5-acetamido-2,6-anhydro-3,5,8-trideoxy-3-fluoro-D-threo-L-galacto-nononic 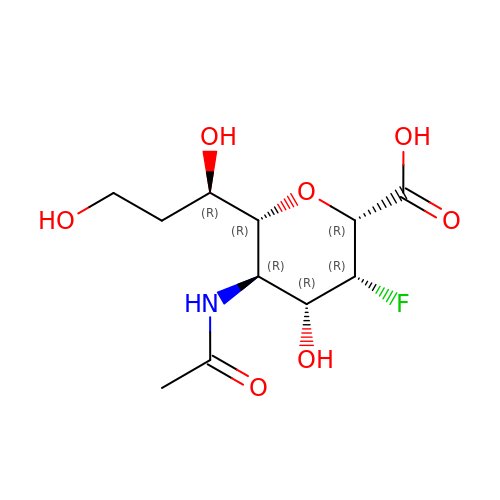acid | C11 H18 F N O7 | MCQSBVLYLCZSNU-AIGBEWNKSA-N> SKPRNQNQVMPLQNVPGWGYSLYKGIDMSVPLAYDPNNELGDLRDVFPSAVDEMAIGYVCGNPAIKHVLTWSTTDVVQNPISNGDDWGGVIPVGMPCYSKTIRAVKG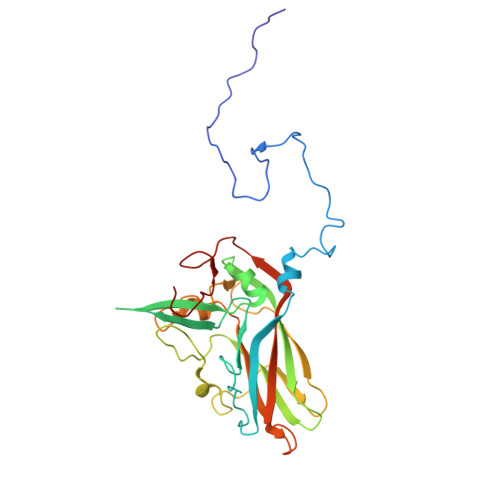ATSTKTEVMDPAPCEYVANLFSYWRATMCYRITVVKTAFHTGRLEIFFEPGSIPTVRTADNLGPDQTQLNGTIAPSDNNYKYILDLTNDTEVTIKVPYVSNKMFMKTVGIYGAHDEDNWNFDESFTGFLCIRPITKLMAPDTVSQKVSIVVWKWAEDVVVVEPKPLTSGPTQVYNPPAVARDL>[2x]MLSEVEFSHEYWMRHALTLAKRAWDEREVPVGAVLVHNNRVIGEGWNRPIGRHDPTAHAEIMALRQGGLVMQNYRLIDATLYV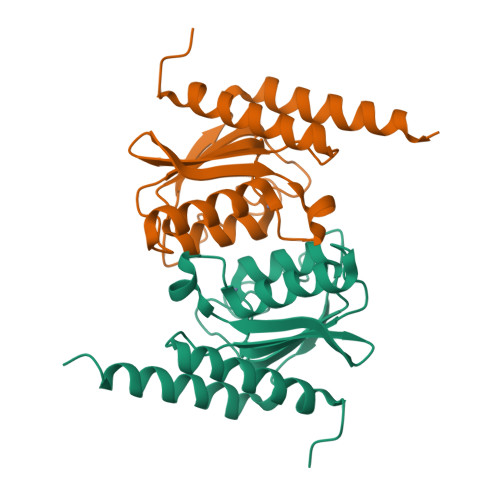TLEPCVMCAGAMIHSRIGRVVFGARDAKTGAAGSLMDVLHHPGMNHRVEITEGILADECAALLSDFFRMRRQEIKAQKKAQSSTD Vesicle amine transport protein-1 (VAT-1) was originally isolated as a synaptic vesicle membrane protein, abundantly found in cholinergic synaptic vesicles, and suggested to be involved in vesicular transport. Although these investigations have suggested a variety of VAT-1 molecular functions in cell regulation, amino acid sequence analysis has indicated that VAT-1 belongs to the NAD(P)-dependent quinone oxidoreductase subfamily. With analysis of the crystal structures of free-form VAT-1 and NADP-bound VAT-1 complex and additional enzymatic studies, we revealed that VAT-1 contains a conserved NADPH binding cleft and binds NADPH to function as an oxidoreductase. VAT-1 comprises ten α-helices (α1–α10), five 310-helices (η1–η5) and sixteen β-strands (β1–β16), and forms two α/β domains, designated as Domain I and II.

We observed clear electron density for the bound NADP molecule. In the NADP-bound form, the nucleotide-binding tunnel is filled by the bound NADP molecule, which adopts an extended conformation and is almost completely buried inside. In the binding tunnel, VAT-1 forms fourteen direct hydrogen bonds with the bound NADP molecule. At one entrance of the tunnel, β9–α5 loop (Ser222), α5-helix (Lys225) and β10–α6 loop (Tyr240, His241) from Domain II form the phosphate-binding site and tightly trap the 2′-phosphate group of ADP moiety by forming six hydrogen bonds with the site, indicating the importance of the 2′-phosphate group of NADPH in VAT-1 binding. The nicotinamide ring forms three hydrogen bonds via the amide group of the nicotinamide with the main chains of β14–η5 loop (Phe326 and Leu328) and the N-terminal end of the Switch segment (Tyr285), whereas the ribose of the NMN moiety has no direct hydrogen bond. NADP binding induces conformational changes in the VAT-1 structure. The major conformational change is found in the Switch segment. On NADP binding, the Switch segment moves from α8-helix of the other protomer, which results in a shift of the protomer (by maximum of ~ 6 Å). We thought that the large empty space on the nicotinamide ring plane in our NADP-bound VAT-1 structure may be the substrate binding site for potential oxidoreductase activity.

>GPASPPLLRCLVLTGFGGYDKVKLQSRPAAPPAPGPGQLTLRLRACGLNFADLMARQGLYDRLPPLPVTPGMEGAGVVIAVGEGVSDRKAGDRVMVLNRSGMWQEEVTVPSVQTFLIPEAMTFEEAAALLVNYITAYMVLFDFGNLQPGHSVLVHMAAGGVGMAAVQLCRTVENVTVFGTASASKHEALKENGVTHPIDYHTTDYVDEIKKISPKGVDIVMDPLGGSDTAKGYNLLKPMGKVVTYGMANLLTGPKRNLMALARTWWNQFSVTALQLLQANRAVCGFHLGYLDGEVELVSGVVARLLALYNQGHIKPHIDSVWPFEKVADAMKQMQEKKNVGKVLLVPGPEKEN[4x]>DYYHATKTTIFNALLNTIDLSQLAQLDLKQAGEEIRDIVAELVAIKNVSMSVAEQEHLVQDIINDVLGYGPLEPLLARDDIADIMVNGAHRVFIEVGGKVQLTNVRFRDNLQLMNICQRIVSQVGRRVDESSPICDARLPDGSRVNVIAPPLALDGPTLTIRKFKKDKLTMKNLVEFASISPEGARVLGVIGACRCNLVISGGTGSGKTTLLNTMTAFIDPTERVVTCEDAAELQLQQPHVVRLETRPPNLEGSGAVTMRDLVKNCLRMRPERIIVGEVRGPEAFDLLQAMNTGHDGSMGTLHANSPREAISRIESMITMGGYGLPSKTIKEMIVGSVDVIIQAARLRDGSRRITHITEVVGLEGDVIVTQDLFVYEITGEDEHGKVVGKHRSTGIARPRFWDRARYYGLERELAEALDAAEA[6x]

The bacterial tight adherence pilus system (TadPS) assembles surface pili essential for adhesion and colonisation in many human pathogens. Pilus dynamics are powered by the ATPase CpaF (TadA), which drives extension and retraction cycles in Caulobacter crescentus through an unknown mechanism. We show that CpaF assembles into a hexamer with C2 symmetry in different nucleotide states. Nucleotide cycling occurs through an intra-subunit clamp-like mechanism that promotes sequential conformational changes between subunits.

After incubation with the non-hydrolysable ATP analogue AMPPNP and in the presence of Mg2+, the sample was vitrified using holey grids and a data set collected for high resolution structure determination. Subsequent data processing yielded a map constituting six subunits arranged in a C2 symmetric ring. Side chain detail was sufficient to build amino acid residues 150–502 relating to the N-terminal domain 2 (NTD2) and C-terminal domain (CTD) for each subunit at 3.8 Å resolution overall. Henceforth, this CpaF structure obtained in the presence of AMPPNP is termed CpaFAMPPNP. Although CpaF was incubated with AMPPNP, this nucleotide was symmetrically bound in only two of the nucleotide-binding pockets within the hexamer. ADP coordinated to a Mg2+ ion (ADP/Mg2+) was symmetrically bound in the neighbouring subunit, with ADP alone in the remaining pair. The ADP is likely derived from AMPPNP hydrolysis given non-hydrolysable ATP analogues are not entirely resistant to hydrolysis. Comparison of the three subunits in the asymmetric unit showed that whilst the AMPPNP and ADP bound chains were relatively similar with RMSD Cα = 1.2 Å, the ADP/Mg2+ chain underwent a significant conformational change where the CTD rotated ~34˚ around Hinge 2. This induced the CTD to swing upwards 18 Å relative to the NTD2 resulting in a clamp-like effect around the nucleotide binding pocket. Importantly, these conformations showcase the key stages in the nucleotide hydrolysis cycle including ATP loading (open state), ATP hydrolysis to ADP with the exit of the γ-phosphate from the active site (closed state), and ADP bound with low affinity primed for release (open’ state).4-[8-azanyl-3-[(3~{R},6~{S})-1-cyclopropylcarbonyl-6-methyl-piperidin-3-yl]imidazo[1,5-a]pyrazin-1-yl]-3-fluoranyl-~{N}-[4-(trifluoromethyl)pyridin-2-yl]benzamide | C29 H27 F4 N7 O2 | 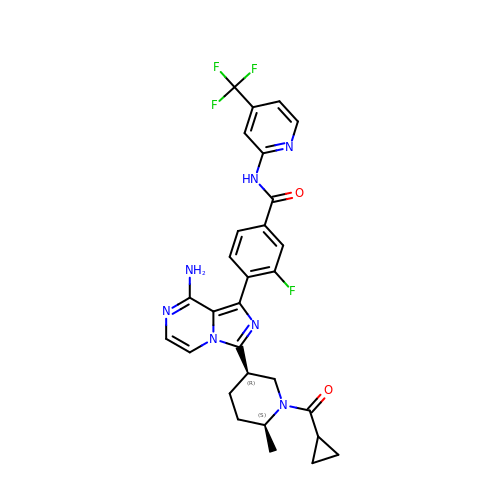JUSWPUDQOKINJO-MAUKXSAKSA-N> ARNGDHCPLGPGRCCRLHTVRASLEDLGWADWVLSPREVQVTMCIGACPSQFRAANMHAQIKTSLHRLKPDTVPAPCCVPASYNPMVLIQKTDTGVS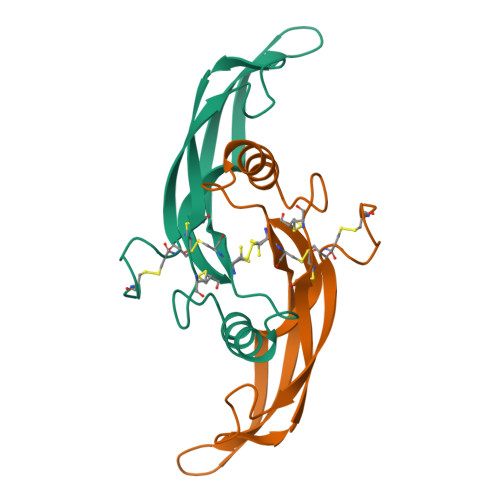LQTYDDLLAKDCHCI>[2x]GPAMGQT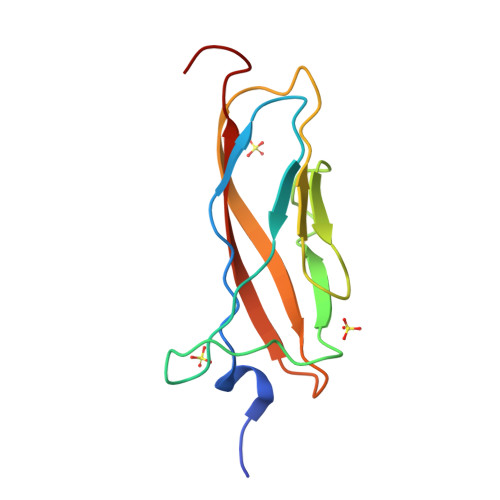ADDHNPKYEDVDVKPGETNKVTPTNTDKDGNPANIPDGTKFEKDPDAPSWVEVDPNTGELTVAPPEGTPSGGHEIKVKVTYPDGSTDEVPVTVKVSDPTTP> GSSGSSGMQAGKPILYSYFRSSCSWRVRIALALKGIDYEIVPINLIKDGGQQFTEEFQTLNP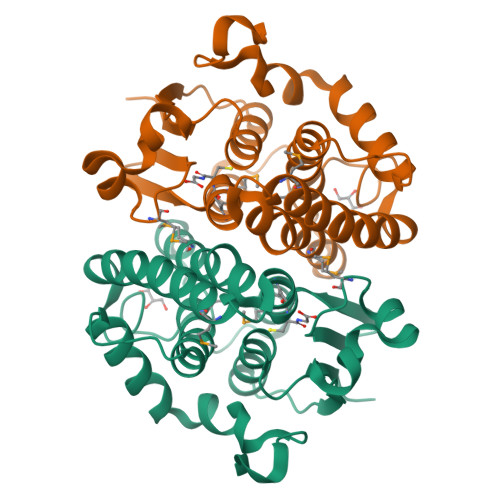MKQVPALKIDGITIVQSLAIMEYLEETRPIPRLLPQDPQKRAIVRMISDLIASGIQPLQNLSVLKQVGQENQMQWAQKVITSGFNALEKILQSTAGKYCVGDEVSMADVCLVPQVANAERFKVDLSPYPTISHINKELLALEVFQVSHPRRQPDTPAELRT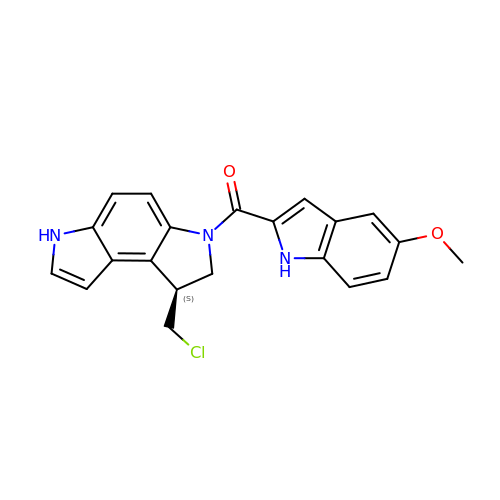[(1S)-1-(chloromethyl)-1,6-dihydropyrrolo[3,2-e]indol-3(2H)-yl](5-methoxy-1H-indol-2-yl)methanone | C21 H18 Cl N3 O2 | ZHFAARVXMYJTEZ-CYBMUJFWSA-N>MGSMATLKAQHLAKSYKGRQVVRDVSMSIDSGQIVGLLGPNGAGKTTCFYMIVGLVQADQGVVRIDEQNVTHLPMHGRARAGIGYLPQEASIFRKLSVSDNIMAILETRSDLDRNGRKEALEGLLQEFHIHHIRDNLGMSLSGGERRRVEIARALASAPKFILLDEPFAGVDPISVGDIKQIIHHLKAKGIGILITDHNVRETLDICETAYIVNDGQLIAEGDAESILANDLVKEVYLGHEFRLKLHHHHHH[2x];> MGSMIVFRYLSREVLVTMSAVSAVLLVIIMSGRFIKYLAQAAQGLLDPGSLFLIMAFRIPGFLQLILPLGLFLGILLAYGRLYLESEMTVLSATGMSQKRLLGYTMAPALLVAILVAWLSLFLAPQGINQFALLLNKQDTLTEFDTLVPGRFQAMRDGTRVTYTEELSKDRGELAGIFISQKDLNSSNQERGISILVAEKGTQNIQADGSRYLILHNGYRYDGNPGQANYRAIQYDTYGVMLPKPEASSEVSERDAVPTADLFGSDNPRYQAELQWRLSTPLLVFVVTLLAVPLSRVNPRQGRFLKLLPAILLYMGYLALLIAVRGQLDKGKIPMAIGLWWVHGLFLAIGLLLFYWEPLRLKLASSRAGREVAHG;> MGSMVKLDRYIGVTVFVAILAVLGVILGLALLFAFIDELNDISASYGIGDALRFIFLTAPRRAYDMLPMAALIGCLVGLGTLASNSELTIMRAAGVSLSRIVWAVMKPMLVLMLAGILVGEYVAPWTENIAQSGRALAQGGGDSQSSKRGLWHRQGREYIHINAVQPNGVLYGVTRYRFDEQRGLESASFAKRARFETDHWQLEEVTTTLLHPREKRSEVVKLPTERWDAQLSPQLLNTVVMEPEALSISGLWQYIHYLADQGLNNNRYWLAFWTKVLQPLVTAALVLMAISFIFGPLRSVTLGQRIFTGVLVGFVFRIAQDLLGPSSLVFDFPPLLAVVIPASICALAGVWLLRRAG

The IM sub-complex comprises the ATP-binding cassette (ABC) transporter LptB2FGC, which extracts LPS from the IM and delivers it to the periplasmic components of the Lpt system. LptB2FGC is a type VI ABC transporter consisting of 5 subunits. The LptB cytoplasmic subunits form the nucleotide-binding domains (NBDs) that capture and hydrolyse ATP. LptF and LptG possess transmembrane helices that create a cavity and a translocation path for LPS, as well as a periplasmic β-jellyroll domain.

Three distinct conformations of LptB2FG, designated as LptB2FG-I, LptB2FG-II, and LptB2FG-III, were captured in our cryo-EM data and solved to resolutions of 3.34 Å, 3.26 Å, and 3.31 Å, respectively. The main difference between the three cryo-EM structures of LptB2FG is in the conformation of the β-jellyroll domain, which appears to perform a rigid body rotation motion with respect to the outer leaflet of the IM, transitioning from one conformational state to the other. The TMD and NBD domains of these three structures are essentially the same. In contrast to all the reported structures of LptB2FG determined by cryo-EM, our cryo-EM structures did not reveal any density consistent with the presence of LPS within the outward-facing cavity of the TMDs. This cavity has a volume of 5,473 Å3, approximately half the volume observed in the X-ray structure (10, 513 Å3), suggesting that the previously solved structure may represent an LPS-bound conformation. Intriguingly, our structures of LptB2FG exhibit an open V-shaped cleft at Interface 1, oriented toward the outer leaflet of the inner membrane, while Interface 2 remains entirely closed. This structural feature is expected to facilitate lipids entering the TMD domain of LptB2FGC via Interface 1. The distinctive structural attributes characterising our cryo-EM LptB2FG structures strongly suggest that we have captured the resting state, or substrate-free conformation, of this transporter. In the LptB2FG-I structure, we observed PE1, PE3, and PE4.> MAAQLALNSEASLWGPYREIWQTVLSALIKRQPEAVHSLDIVLKKYKPDFISLFKNPPKSAQQHERVQKASTEGIPIKGTQRTRILEEQLIKEAFILSDLYNIGEIAAVELLLIGEQQQPTFHGLTRGLVAILLYWDGKSCMAESLLHLIQARKGKTFTLDHSPEVVSMVTRFTDDLMEQGLTNKILTLISQIDVNNEFDKLKKERGLGNKKHRKEVSDLIKECQQSLAHSLYSWSCQTPLNREDTLLLIGYLEKVTVEGDGSLDKVNLTLLMSLLYCLDVGFLEQGTDDREELMKQASMFMDRQYIAAIHNRLQNTQPWKSPGMQATVRLAWALALRGISQFSEVLEFSEADEPMAEIAIGGNVFLFLTEAVVGSESFCTDEFFIRRIHKLVTDFPTLMPMKVKQLRNRAEEDARLIQMSMQMGNEPPASLRRDLEHLLLLIGELYRKDPFHLELALEYWCPTEPLQSTSLMGSFLGVAHQRPPQRQVLLSKFVRQMSDLLPATLYLPYLKMLRGLASGPQCAHYCFSLLKANGGSSAENLQAAGGSPVSWDHFFHSLMLYHEHLRRDLPNTDNIHQRHPPLRGITQRELDGLIACLQLTCTIIDWSESARLALCEHAQWMPVVVILGLLQCSIPPLLKAELLKTLAAFGKSPEIAASLWQSLEYTQILQTVRATGLRQGVGIEVELNEIESRCEEYPLTRAFCQLISTLV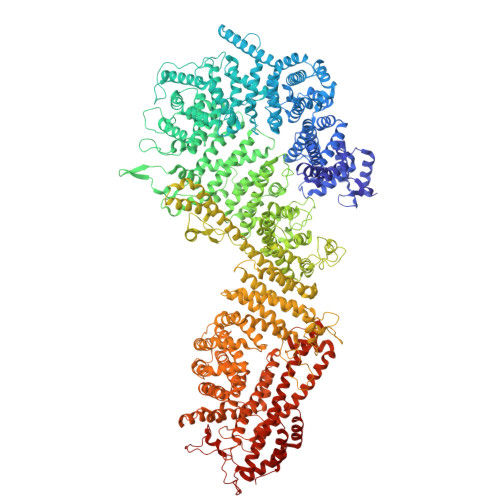ESSFPTNLGAGLRAPGFEPYLQFLRDTVFLRYRTRAYRRAAEKWEVAEAVLDVFYKLLKDYEPQPEDFVDQYVELQGEERVAFKPPGFSLMHHLLNESPMLELCLSLMEEGVTQLDTYAPFPGKKHLEKAVAYCFMLLNLTLQKENRFMDLLRESHLSMIVTPLEQLLQGINPRSKKADNVVNIARYLCHGNSNAELAFESAKILCSISCNSKIQEKIVGDFTQDQNVSQKLMVGFVSCLDSEEAEELLDSEKEAEDQVKQTNIRYMTKIHILNLLITSLEMKAPNLAMFLLGYELKKPVSTTNLQDSGVLGCPRTCLHSILDILRKGTDVRAGPVAVWDTPHLAELCYQVIYQLCACADTSGPTMRYLRTSQDFLFSQLQHLPFSVEESEISAMNQMSWLMKTATIELRITSLNRQRSHTQRLLHLLLDDMPTRPYSADGEGGMEDESRSLSGFLHFDTTSKVRRKILRILDSIQFSNEIPEPLQLDFFDRSQIEQVIANCEHKNRRGQTVCNVKLLHRVLVAEVNALQGMAAIGQRPLLMEEINTILQYVVERNKLLQCLHAKRHALESWRQLVEIILTACPQDLIPTEHRQLIIRDLLQDLHVKILDDDAAQELMPIVAGAVFTLTAHLSQSVRTELKQPMTASGLGQSQYVQMLDGSFAAPPGTENISAGFASIGDSSLHMILRNLLEFILKTGGGFQRVRAHLYGSLLYYLQIAQRPDEPDTLESAHKSMWERLTAPEDVFSKLQRDNLSIFESYGTALMEVVCRDACDGHDIGRMLALALLDRIVSVDRQQQWLLYLSNSGYLKVLVDSLAEDDVVLRNLLTPQPPLLKALYIYESKMAFLTRVAKSSQGAIELLRSGVIVRLAQCQVYDMRPETDPHGVFGMRETPVFIPAPVERYRQILLPALQICQLILTSSTAQHLQAAGQVLQFLVAHSDTIQAILRSQEGSLGSLQELALLTGIISKAALPGVLNELDIGLNDGSMMELQGHIGRFQRQCLALLNRFGGSDRLRQLSLQDDSSRLDGVSKKDDMELAMQQICSNVMEYCQALMIQNSPSFQQTVCLFTPSLKESASRDGTRQDSQVSILPSWRLPSLGVVIHLLKQSANNFFTYYDIHRQSVGKLQNVEQLPPDEIKELCQSEMPVGADKISTTQKYGLARRRLVKLINSRAKLLSLCSYIIETCLYILWRHLEYYLLHCTTSDSQDPVFSNMTFGNRRFQDTFNTDPNMDPRNLRQNKVSQQDVDTLLREGANSFGESLQKRLLDIESLYCKVRSRHSFIQALVRRIRGLLRVSRV>[2x]MEILYTGASESLHSTILKALLERIDLGDTFISDNYTRWQATERYYMMYKIPNKKDKAAIEKWNKGDTDFKSLVMPYSYAQLMTAHAYMVNVFLNRDPIFQTDSLNGDGTERELALESMLQYQVKAGEMEPSLLVWFMDALRYGVGVLGDYWEEHVFHQTVFEEEEEIIDGVPTGNMKKVKKTRVVKGYEGCKTFNVMVYDFIPDPRVALCKYQEGEFFGRRLDLNVLDLKKGAKFGKYFNVEHAEALVAASKEEMYRRDPSIGQQRSLKDSTMTPKGKQVGDISCVEIFVRLVPKDWGLGDSEFPEMWVFTVADKKYIVAAEPVNTLDDKFPFHILECEIDGYMNKSRGLLEISAPMNDILTWLFDSHMYNKRQIMNNQFIGDPSALVVKDVESKEPGKFIRLRPTAYGRDVRSIISQLPVTDVTAQNIQDVQVVERNMQRIVGVNDDVAGQSSPSSRRSATEFRGTTSFASSRLANLAYFFSVTGFRSLAKSLIVKTQQLYTVEMKVKVAGDNIKGAQSIIVKPEDISGQFDIMPVDGTLPVDRMAQAQFWMQIMSMVAGNPVLGAEYRLGDIFSYTARLAGLKGIDKMKIRILDDDQILALILAQQKGGADVQPTGQPTTQGVGNPTGVNEPAPSVTQGTPGLSGLQALM;>MDKATLVKTIAYRMGNVKGQDTAIDFELALSIERLEGQEFVPWFLLSENNFFEGTAQENR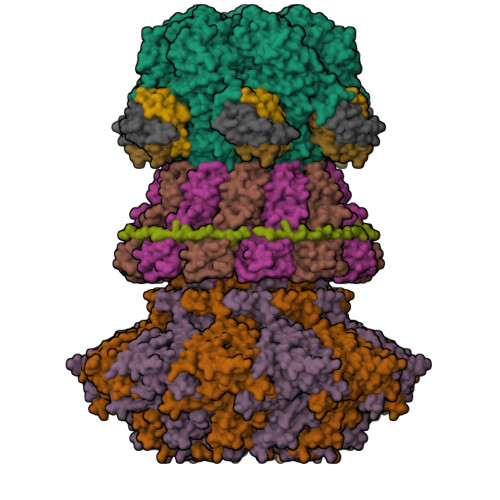IPVPRGFIREYEEGSLYLRRVAGTGKCLIKKSQDQLLKYEGMTGEPSHYSLTNQYFRIYPVPQEDFKVELLFYRKSSTLNVEDNPWYEYAAELLVAETIWAMLSARRDKMADYWKSVAADQMRRLTILDAERRLANQEIFMG[2x];> MEVTHKQFDLSGFLPDQAPDTLKSGAISRGFNVKPTILGWEKSGGFRETNTAPTNEKDFIFFWSPAIGDNRWFSGGDKTVQQVEGNVVSDVSRTGGYTAGSGRRWNAVNFNGVLLMNNELDSPQYLAASGKLEDFPNLPSNVRFRTVAVYKNFILGLGVNFGSGFLDDEIYWSHQADPGTMPPNWDYANAASDSGRTPLPSEGYCVTSEELGSMNIVYKSDSIWTMQLIGGQWIFRFENKFPGQGILNKKSVVSFEGKHFVVTQKDIIVHDGYQVRSVADKRVRNFFFTDMNSDYFERVFVVKDPRVAEVYVFYPSKNSVDGLCDRALVWNWRDDVWSLLNLRPLKHAAYGYEITGVSITWDNFVGGWESTGLWQADEDVAKYAPVLHYSFRDVPKLLAPTPQALFIDEEIEAVWEREDIVIGSISRDGVPYQDYERNKSVSSISFDVDTTEPFDVYIGYKGSLEDSVEWEFAGTVNPMEDKRLFCLLTAGLFSMRIISKAQTFILRSYKITYEFAGEMWS;> MSSWDRFDTPWDSIIDESTWEHYTFKYDASFEAFSSMEVDEDLTITVSVLFASTSDNTVTVGQVLGLTMDNRAGSYFGAGSSWTSEAAVNNEAGSGFQSSHALQLSYSVEDGVISSFGSEAFCSFYNTVSFESSSDVQAAVNSLYNLDVLFSSGSGDSEQHYVVFGETASFESLAEHETSSQYITHVECMFNSVVEFEVKTYDWGRPVKPVGSDWSTDTPVVGVWVNEIYNGNKDWGES;>MALETWDANSTPATLNTAWPEATDPLNKGDDHIRLLKTVVVNFWNKVFDGSKLKTAVVPAAVNSATAGSGFGGFRYQVVNNSDGTKTLRLFTS[3x]> STKDFNLDLVCVSKKDSGASPRITXIS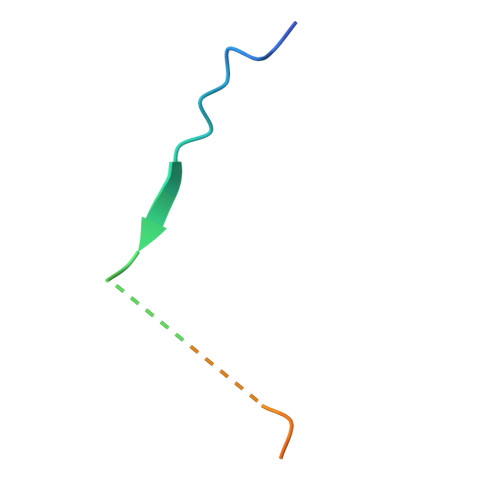LATPGAK(1S,2S,3S,4R,5R)-2-[(cyclopropylmethyl)amino]-4-(phenylsulfanyl)-6,8-dioxabicyclo[3.2.1]octan-3-ol | C16 H21 N O3 S | 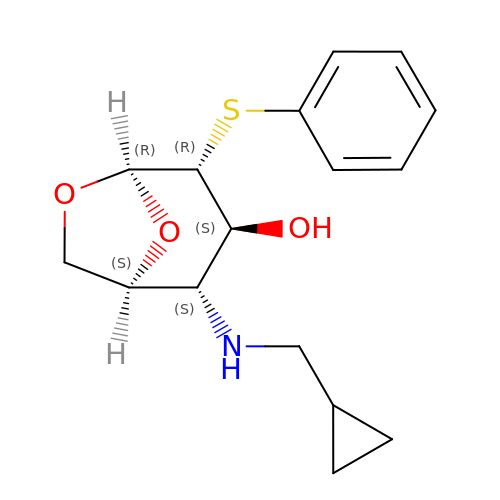RHZAVNISDMVYNF-IBEHDNSVSA-N>[3x]MRIGEWMRGLLLCAGLMMCGVVHADISTVPDETYDALKLDRGKATPKETYEALVKRYKDPAHGAGKGTMGDYWEPIAISIYMDPNTFYKPPVSPKEVAERKDCVECHSDETPVWVRAWKRSTHANLDKIRNLKSDDPLYYKKGKLEEVENNLRSMGKLGEKETLKE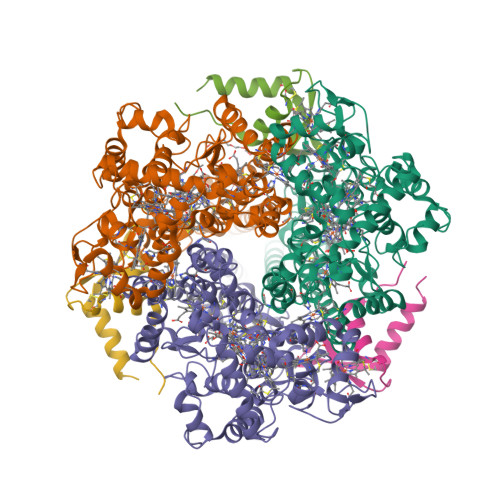VGCIDCHVDVNKKDKADHTKDIRMPTADTCGTCHLREFAERESERDTMVWPNGQWPAGRPSHALDYTANIETTVWAAMPQREVAEGCTMCHTNQNKCDNCHTRHEFSAAESRKPEACATCHSGVDHNNWEAYTMSKHGKLAEMNRDKWNWEVRLKDAFSKGGQNAPTCAACHMEYEGEYTHNITRKTRWANYPFVPGIAENITSDWSEARLDSWVLTCTQCHSERFARSYLDLMDKGTLEGLAKYQEANAIVHKMYEDGTLTGQKTNRPNPPEPEKPGFGIFTQLFWSKGNNPASLELKVLEMAENNLAKMHVGLAHVNPGGWTYTEGWGPMNRAYVEIQDEYTKMQELSALQARVNKLEGKQTSLLDLKGTGEKISLGGLGGGMLLAGALALIGWRKRKQTRA;>[3x]MNKVIVAAFVSAFVLGSTATFASGNLESSLAPISAKDMLDYLACKDKKPTDVVKSHTEVENGKIVRVKCGDIVALVQKAREQSGDAWQGGY>MASVHGTTYELLRRQGIDTVFGNPGMNELPFLKDFPEDFRYILALQEACVVGIADGYAQASRKPAFINLHSAAGTGNAMGALSNAWNSHSPLIVTAGQQTRAMIGVEALLTNVDAANLPRPLVKWSYEPASAAEVPHAMSRAIHMASMAPQGPVYLSVPYDDWDKDADPQSHHLFDRHVSSSVRLNDQDLDILVKALNSASNPAIVLGPDV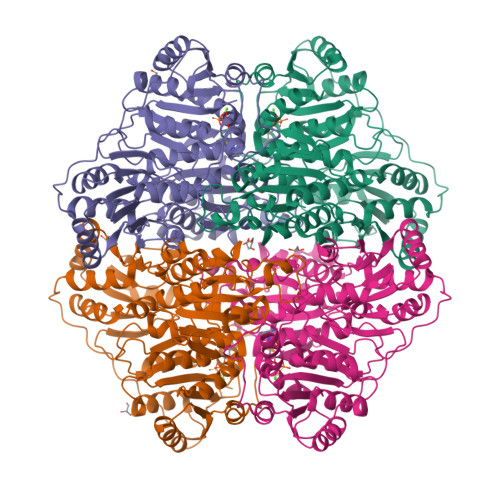DAANANADCVMLAERLKAPVWVAPSAPRCPFPTRHPCFRGLMPAGIAAISQLLEGHDVVLVIGAPVFRYHQYDPGQYLKPGTRLISVTCDPLEAARAPMGDAIVADIGAMASALANLVEESSRQLPTAAPEPAKVDQDAGRLHPETVFDTLNDMAPENAIYLNESTSTTAQMWQRLNMRNPGSYYFCAAGGLGFALPAAIGVQLAEPERQVIAVIGDGSANYSISALWTAAQYNIPTIFVIMNNGTYGALRWFAGVLEAENVPGLDVPGIDFRALAKGYGVQALKADNLEQLKGSLQEALSAKGPVLIEVSTVSPVKHHHHHH[4x]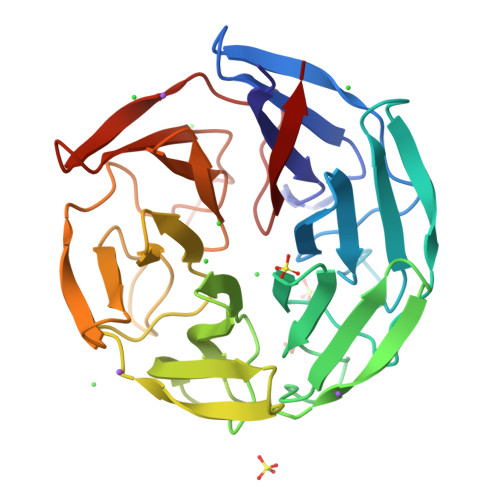>[2x]GAGPVLFAVGGGSLFAIHGDCEAYDTRTDRWHVVASMSTRRARVGVAAVGNRLYAVGGYDGTSDLATVESYDPVTNTWQPEVSMGTRRSCLGVAALHGLLYSAGGYDGASCLNSAERYDPLTGTWTSVAAMSTRRRYVRVATLDGNLYAVGGYDSSSHLATVEKYEPQVNVWSPVASMLSRRSSAGVAVLEGALYVAGGNDGTSCLNSVERYSPKAGAWESVAPMNIRRSTHDLVAMDGWLYAVGGNDGSSSLNSIEKYNPRTNKWVAASCMFTRRSSVGVAVLELL>[3x]QGILSLALKDKAALYSAYMPFVKSGGIFVPTPKRYMLGDEVFLLLTLPDS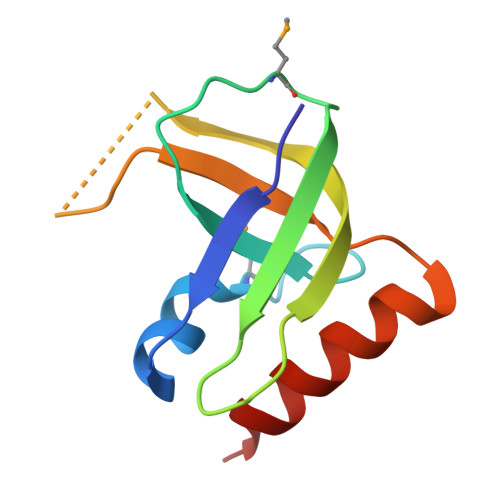SERLPVAGKVVWTTPAGAQGNRAAGIGVQFPDGPEGEAVRNKIETLLAG>NLIPTVIEQTNRGERAYDIYSRLLKDRIIMLGSAIDDNVANSIVSQLLFLAAEDPEKEISLYINSPGGSITAGMAIYDTMQFIKPKVSTICIGMAASMGAFLLAAGEKGKRYALPNSEVMIHQPLGGAQGQATEIEIAAKRILLLRDKLNKVLAERTGQPLEVIERDTDR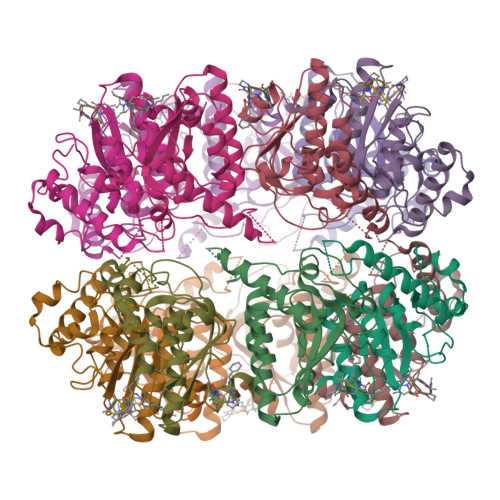DNFKSAEEALEYGLIDKILTHTEDKKHHHHHH[14x];>[14x]XFSPAAP> GSNVLTVYSPYQSNLIRPILNEFEKQEHVKIEIKHGSTQVLLSNLHNEDFSERGDVFMGGVLSETIDHPEDFVPYQDTSVTQQLEDYRSNNKYVTSFLLMPTVIVVNSDLQGDIKIRGYQDLLQPILKGKIAYSNPNTTTTGYQHMRAIYSMHHRVSDVHQFQNHAMQLSKTSKVIEDVAKGKYYAGLSYEQDARTWKNKGYPVSIVYPIEGTMLNVDGIALVKNAHPHPKRKKLVQYLTSRSVQQRLVAEF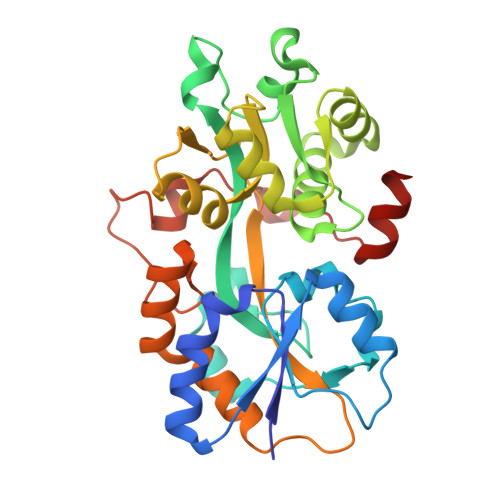DAKSIRKDVSEQSDQSIENLKNIPLIPKSKLPDIPHHKFLEMIQ>[2x]MRGSFANDATFEIKKCDLHRLEEGPPVTTVLTREDGLKYYRMMQTVRRMELKADQLYKQKIIRGFCHLCDGQEACCVGLEAGINPTDHLITAYRAHGFTFTRGLSVREILAELTGRKGGCAKGKGGSMHMYAKNFYGGNGIVGAQVPLGAGIALACKYNGKDEVCLTLYGDGAANQGQIFEAYNMAALWKLPCIFICENNRYGMGTSVERAAASTDYYKRGDFIPGLRVDGMDILCVREATRFAAAYCRSGKGPILMELQTYRYHGHEMSDPGVSYRTREEIQEVRSKSDP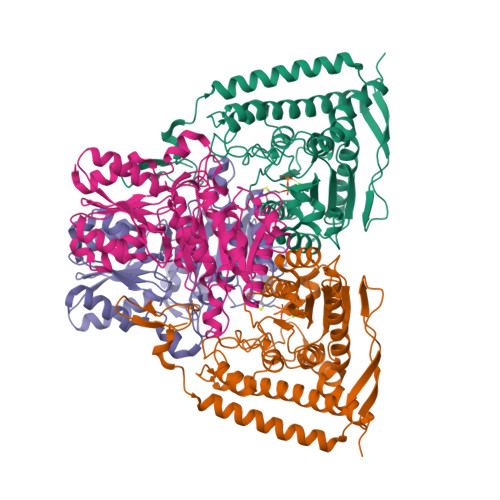IMLLKDRMVNSNLASVEELKEIDVEVRKEIEDAAQFATADPEPPLEELGYHIYSSDPPFEVRGANQWIKFKSVS;>MRGSHHHHHHGSLQVTVRDAINQGMDEELERDEKVFLLGEEVAQYDGAYKVSRGLWKKYGDKRIIDTPISEMGFAGIAVGAAMAGLRPICEFMTFNFSMQAIDQVINSAAKTYYMSGGLQPVPIVFRGPNGASAGVAAQHSQCFAAWYGHCPGLKVVSPWNSEDAKGLIKSAIRDNNPVVVLENELMYGVPFEFPPEAQSKDFLIPIGKAKIERQGTHITVVSHSRPVGHCLEAAAVLSKEGVECEVINMRTIRPMDMETIEASVMKTNHLVTVEGGWPQFGVGAEICARIMEGPAFNFLDAPAVRVTGADVPMPYAKILEDNSIPQVKDIIFAIKKTLNI[2x]> LRVQPEAQAKVDVFREDLCTKTENLLGSYF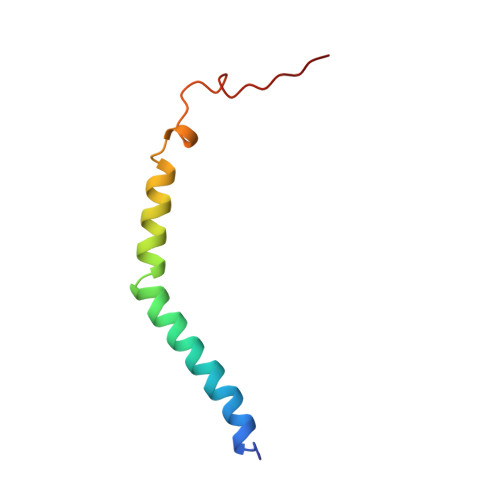PKKISELDAFLKEPALNEANLSNLKAPLDI>[2x]GMNVNFINPFLQSLLNVISTMA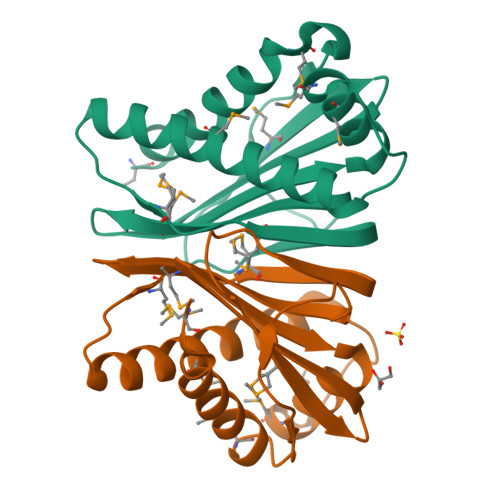SLELTPGKPQIKTDNLAKGDVSGLIGMVGPQTKGSLSITFEQKLVLQIMQNMLGENPGKINEEVTDLVGEITNMVTGGAKNLLGQKGYEFEMATPMVVSGQGHTISHKANGTKIIMPFTSSYGTAFIEVCFES3-fluoro 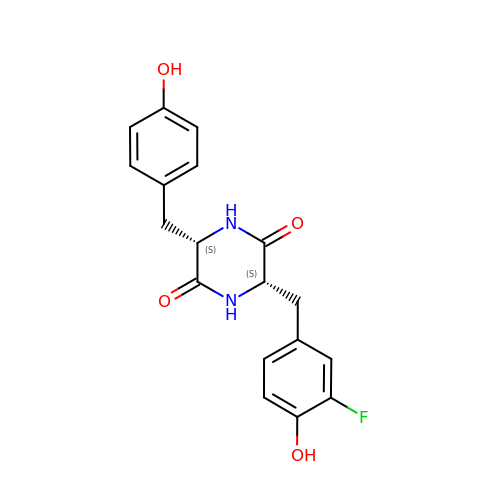dicyclotyrosine | C18 H17 F N2 O4 | BWLHGYWAFIMGJI-GJZGRUSLSA-N> GPLGSMANRDDIDASAVMAAYLAREYAEAVEEQLTPRERDALEALRVSGEEVRSPLLQELSNAGEHRANPENSHIPAALVSALLEAPTSPGRMVTAVELCAQMGRLWTRGRQLVDFMR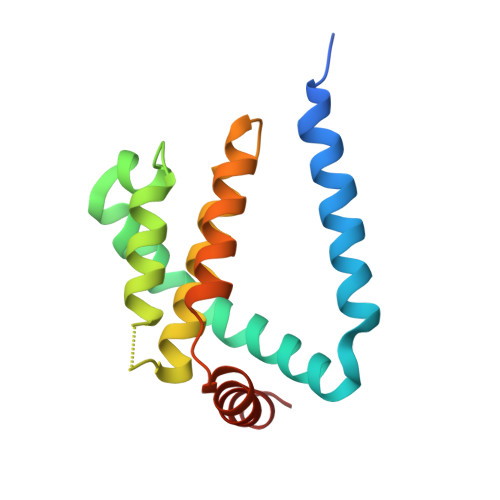LVYVLLDRLPPTADEDLGAWLQAVARVHGT> HTEILRGLRFTLLFVQHVLEIAALKGSASEAAGGPE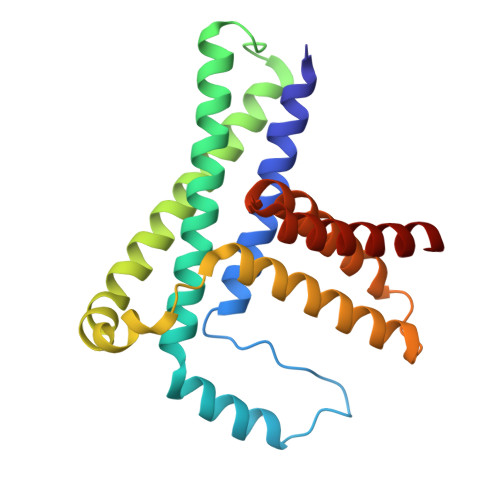YQLQESVVADQISLLSREWGFAEQLVLYLKVAELLSSGLQSAIDQIRAGKLCLSSTVKQVVRRLNELYKASVVSCQGLSLRLQRFFLDKQRLLDRIHSITAERLIFSHAVQMVQSAALDEMFQHREGCVPRYHKALLLLEGLQHMLSDQADIENVTKCKLCIERRLSAL>[2x]YVEGQRKRRNTIHEFKKSAKTTLIKIDPALKIKTKKVNTADQCADRCTRNKGLPFTCKAFVFDKARKQCLWFPF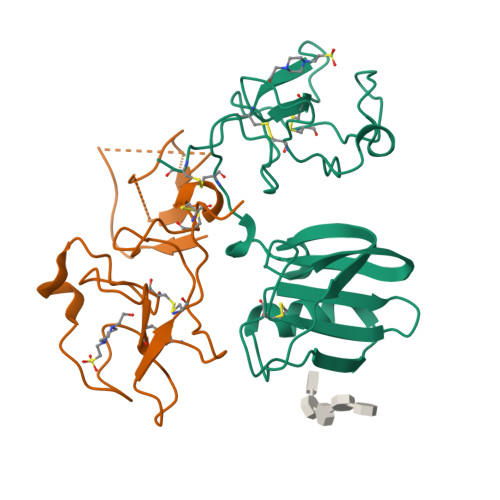NSMSSGVKKEFGHEFDLYENKDYIRNCIIGKGRSYKGTVSITKSGIKCQPWSSMIPHEHSFLPSSYRGKDLQENYCRNPRGEEGGPWCFTSNPEVRYEVCDIPQCSEVE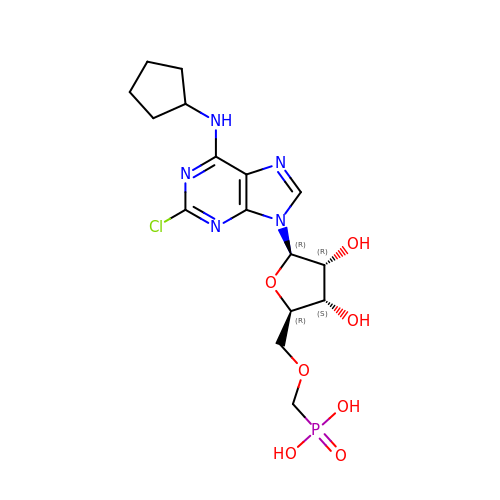[(2~{R},3~{S},4~{R},5~{R})-5-[2-chloranyl-6-(cyclopentylamino)purin-9-yl]-3,4-bis(oxidanyl)oxolan-2-yl]methoxymethylphosphonic acid | C16 H23 Cl N5 O7 P | ALDWNWOVOJESRL-SDBHATRESA-N>[2x]GPHMASLVIISTLDGRIAALDPENHGKKQWDLDVGSGSLVSSSLSKPEVFGNKMIIPSLDGALFQWDRDRESMETVPFTVESLLESSYKFGDDVVLVGGKSLTTYGLSAYSGKVRYICSALGCRQWDSDEMEQEEDILLLQRTQKTVRAVGPRSGNEKWNFSVGHFELRYIPDMETRAGFIES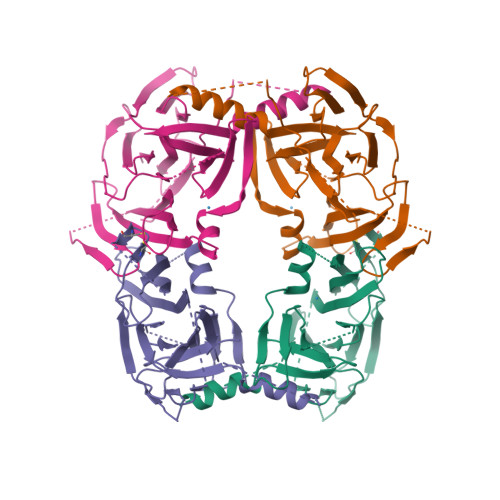TFKPNENTEESKIISDVEEQEAAIMDIVIKVSVADWKVMAFSKKGGHLEWEYQFCTPIASAWLLKDGKVIPISLFDDTSYTSNDDVLEDEEDIVEAARGATENSVYLGMYRGQLYLQSSVRI>MGSSHHHHHHSQDLEVLFQGPGSQRRYALQAHQD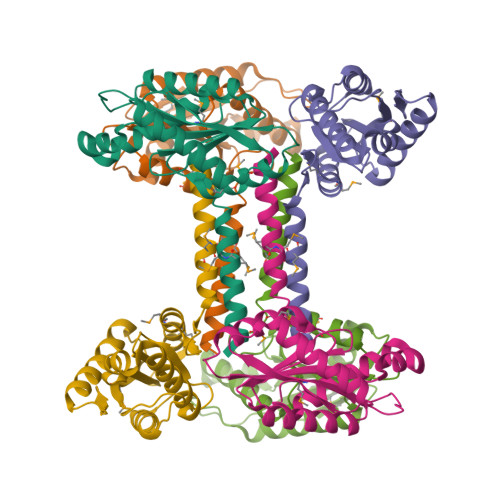TLRGMMRQLEDLVATDELTGLFNRRHFMRMASRALEDLLPNRQHGLALIDLDHFKRINDRHGHAAGDRVLQTFAAVARSCLRDGDVLARYGGEEFVLLLPHADAEQLESCCERLRLAFQQAEPVGVTVDTLSLSVGMTLLYADDDLDEALQRADQALYRAKRGGRNRCDATWEVTSA[3x]>MLQCYNCPNPTADCKTAVNCSSDFDACLITKAGLQVYNKCWKFEHCNFNDVTTRLRENELTYYCCKKDLCNFNEQLE[6x];>XYSWTWGNRSSVRGCX[3x]

CD59 is a cell surface protein that plays an important role in mediating human health and disease. CD59 is the only membrane‐bound inhibitor of the complement‐mediated membrane attack complex (MAC), and it is the body's last line of defense against MAC‐mediated cell death. CD59 directly binds the alpha chain of C8 (C8α) as the β‐hairpins cascade toward the membrane and sterically blocks the transmembrane residues of C9 from accessing the membrane, inhibiting pore formation. In contrast to its role inhibiting MAC pores, CD59 may be hijacked by cholesterol‐dependent cytolysins secreted by Gram‐positive bacterial pathogens, which use CD59 as a receptor on human cells to promote oligomerization of toxins at the membrane.

Crystals of CP‐06 in complex with the ectodomain of CD59 diffracted to 2.4 Å, and the structure was solved by molecular replacement. In the crystal structure, two CD59 molecules sandwich a single macrocyclic peptide, with three sets of complexes in the asymmetric unit. The macrocyclic peptide forms a β‐hairpin that is stabilized on each side by an extensive network of hydrogen bonds between C‐terminal β‐strands of the adjacent CD59 molecules. Together they create a large antiparallel intermolecular β‐sheet, in which the two copies of CD59 are oriented in opposite directions. The unique geometry of the d‐Tyr1 within the cyclic peptide facilitates the β‐turn at the tip of the hairpin, consistent with a known role for d‐amino acids in structuring short β‐hairpins. Furthermore, the cross‐strand pairing of Trp3 with Gly13 also likely contributes to peptide secondary structure, while Asn7, Arg8 of the GNR motif, and Ser9 form the second β‐turn of the cyclic peptide. Despite an extensive H‐bond network with backbone atoms, there are no hydrogen bonds between side‐chain atoms of CD59 and CP‐06. Instead, side‐chain interactions are dominated by hydrophobic contacts involving CD59:F47, T60, L59, Y61, Y62, and F42. Specifically, the CD59:Y62 side chain intercalates between the peptide Trp3 and Trp5 residues and explains the significant reduction in binding when either peptide residue is substituted for Ala. Despite a lack of sequence homology between CP‐06 and the β‐hairpin binding motifs of C8α and ILYd4, CD59 residues CD59:F47, CD59:Y61, CD59:Y62, and CD59:E58, which dominate the CP‐06 interface, contribute to both MAC and bacterial toxin binding modes.> MKQKVHSVSYLAKAEFKFNNGVYNLVALPSGAEVVKVSLEVVGNPIAT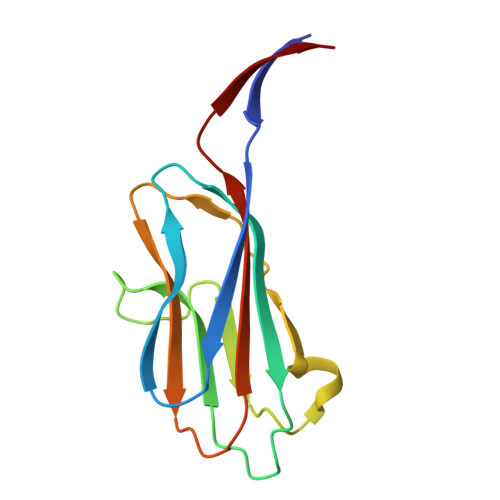STTSVSVGFEDETTKNYFLTLDNLAVDDASKKHTTSAKDYTATSNKVVVAEVKNANDNNVKGVLRVLYFLPSVIEVEY>MNHKVHMKNIQVVVRCRPFNLAERKASAHSIVECDPVRKEVSVRTGGLADKSSRKTYTFDMVFGASTKQIDVYRSVVCPILDEVIMGYNCTIFAYGQTGTGKTFTMEGERSPNEEYTWEEDPLAGIIPRTLHQIFEKLTDNGTEFSVKVSLLEIYNEELFDLLNPSSDVSERLQMFDDPRNKRGVIIKGLEEITVHNKDEVYQILEKGAAKRTTAATLMNAYSSRSHSVFSVTIHMKETTIDGEELVKIGKLNLVDLAGSENIGRSGAVDK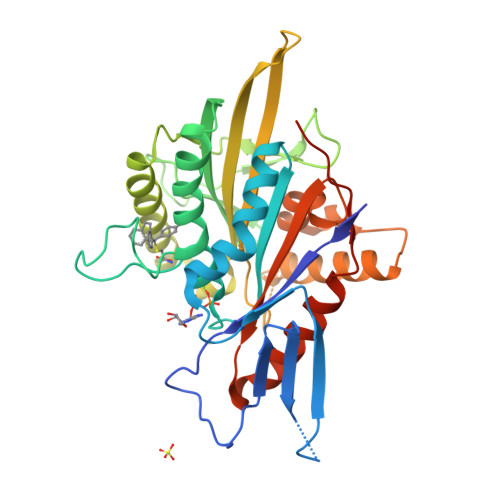RAREAGNINQSLLTLGRVITALVERTPHVPYRESKLTRILQDSLGGRTRTSIIATISPASLNLEETLSTLEYAHRAKNILNKPEVNQKLQHHHHHH[2x]> MVPAESNAVQAKLAKTLQRFENKIKAGDYYEAHQTLRTIANRYVRSKSYEHAIELISQGALSFLKAKQGGSGTDLIFYLLEVYDLAEVKVDDISVARLVRLIA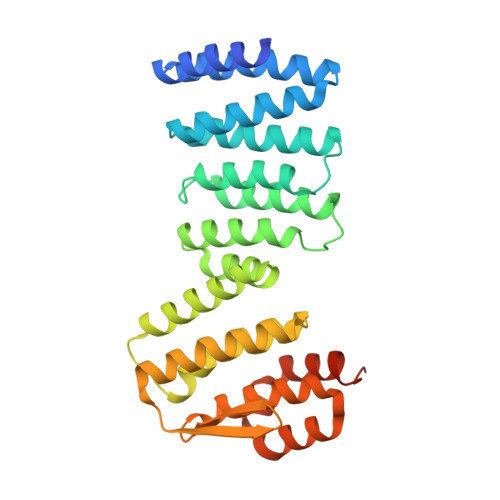ELDPSEPNLKDVITGMNNWSIKFSEYKFGDPYLHNTIGSKLLEGDFVYEAERYFMLGTHDSMIKYVDLLWDWLCQVDDIEDSTVAEFFSRLVFNYLFISNISFAHESKDIFLERFIEKFHPKYEKIDKNGYEIVFFEDYSDLNFLQLLLITCQTADASYFLNLKNHYLDFSQAYKSELEFLGQEYFNENLYFQSLEHHHHHH> GHMKQEELKRLYKAQAIQRQLEEVEERQRASEIQGVRLEKALRGEADSGTQDEAQLLQEWFKLVLEKNKLMRYESELLIMAQELELEDHQSRLEQKLREKMLKEESQKDEKDLNEEQEVFTELMQVIEQRDKLVDSLEEQRIREKAEDQHFES;> GHMNPEYDYLFKLLLIGDSGVGKSCLLLRFADDTYTESYISTIGVDFKIRTIELDGKTIKLQIWDT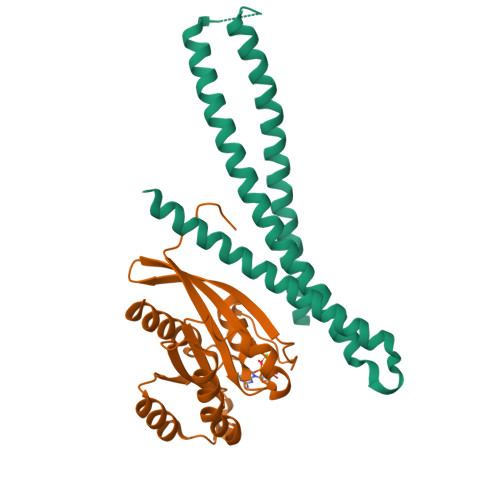AGQERFRTITSSYYRGAHGIIVVYDVTDQESYANVKQWLQEIDRYASENVNKLLVGNKSDLTTKKVVDNTTAKEFADSLGIPFLETSAKNATNVEQAFMTMAAEIKKRMGPGAASGGERPNLKIDSTPVKPAGGGCC Members of the presynaptic neurexin (NRX) and postsynaptic neuroligin (NL) transmembrane protein families form the axis of a signaling pathway that is crucial for the formation and function of excitatory and inhibitory synapses throughout the brain. MDGA proteins bind NLs and control their function and interaction with NRXs via unknown mechanisms. MDGA proteins are attached to the postsynaptic membrane via a C-terminal GPI anchor, and their large (∼900 amino acids) extracellular domain consists of six immunoglobulin-like domains (Ig1-6), a fibronectin type III-like (FnIII7) domain, and a memprin, A5, mu (MAM8) domain. The extracellular region of the NLs contains a cholinesterase-like domain that forms a stable interaction with the α/β-NRX1-3 LNS6 (laminin, NRX, sex-hormone-binding globulin) domain (Araç et al., 2007, Chen et al., 2008, Fabrichny et al., 2007).

We performed an extensive crystallization screening of the NL-MDGA complexes formed between MDGA1-2ECTO and NL1-2ECTO constructs from various species, and succeeded in generating diffraction-quality crystals and determining the structure of the Endo F1-treated complex formed between cMDGA1ECTO and the human NL1 cholinesterase domain lacking splice inserts (hNL1ECTO; Gln46-Asp635) at 3.30 Å. The hNL1ECTO-cMDGA1ECTO complex has a 2:2 stoichiometry and overall dimensions of ∼180 Å wide, ∼110 Å high, and ∼120 Å deep. Two MDGA1 monomers flank the NL1 dimer to form a 2-fold symmetric complex. The NL1 and MDGA1 C termini point in the same direction and thus confirm an interaction in cis, situated on the postsynaptic membrane. Each MDGA1 molecule spans the NL1 dimer using two large, separate interaction sites located on both NL1 monomers (Sites I and II). The Ig1-3 domains mediate all MDGA1 contacts, consistent with previous domain-deletion experiments (Pettem et al., 2013). The smaller Site I (859 Å2 BSA) is formed between residues from (1) MDGA1Ig1 β strands C, F, and G and loop CE and (2) NL1 loops Leu289-Gln307, Ile377-Asp385 (part of “loop L1”), Gln392-Tyr398, and Phe496-Pro499 and helices α2(4,5) and α4(6,7). The larger Site II (1,000 Å2 BSA) is formed between residues from MDGA1Ig2 β strands A, B, D, and E and NL1 α helices α2(7,8) and α3(7,8); (2) MDGA1Ig2 loop ABIg2 and NL1 loops Ala110-Pro132 (“Cys loop”) and Asp361-Asp385 (“loop L1”); and peripheral interactions contributed by MDGA1Ig3 to NL1 α helix α2(7,8) and loop Val417-Ser424. The PheNL1430-PheMDGA1154 π-π sandwich stacking interaction is central to this interface and is lined by multiple hydrogen-bonding and charged interactions. Furthermore, the LRE motif is present in the majority of mammalian AChEs, and besides in NL, it is also observed in the cholinesterase-like adhesion molecules neurotactin and glutactin. Both Arg450 and Glu451 form an integral part of the NL-MDGA interface and interact with Tyr187 and Leu190, respectively, on MDGA1 loop DEIg2, offering a first functional role for this LRE-tripeptide in NLs.

> TGQKLDDVDPLVATNFGKIRGIKKELNNEILGPVIQFLGVPYAAPPTGERRFQPPEPPSPWSDIRNATQFAPVCPQNIIDGRLPEVMLPVWFTNNLDVVSSYVQDQSEDCLYLNIYVPTEDDIRDSGGPKPVMVYIHGGSYMEGTGNLYDGSVLASYGNVIVITVNYRLGVLGFLSTGDQAAKGNYGLLDLIQALRWTSENIGFFGGDPLRITVFGSGAGGSCVNLLTLSHYSEGLFQRAIAQSGTALSSWAVSFQPAKYARMLATKVGCNVSDTVELVECLQKKPYKELVDQDIQPARYHIAFGPVIDGDVIPDDPQILMEQGEFLNYDIMLGVNQGEGLKFVENIVDSDDGISASDFDFAVSNFVDNLYGYPEGKDVLRETIKFMYTDWADRHNPETRRKTLLALFTDHQWVAPAVATADLHSNFGSPTYFYAFYHHCQTDQVPAWADAAHGDEVPYVLGIPMIGPTELFPCNFSKNDVMLSAVVMTYWTNFAKTGDPNQPVPQDTKFIHTKPNRFEEVAWTRYSQKDQLYLHIGLKPRVKEHYRANKVNLWLELVPHLHNLNDRTKHHHHHH;> QGVYAPAQAQIIHAGQACVVKEDNISERVYTIREGDTLVLQCLVTGHPRPQVRWTKTAGSASDKFQETSVLNETLRIEKIQRLQGGRYYCKAENGVGVPAIKSIRVDVQYLDEPVLTVHQTISDVRGSFYQEKTVFLRCTVNSNPPARFIWKRGAETLSHSQDNGVDIYEPLYTQGETKVLKLKNLRPQDYASYTCQVSVRNVCSIPDKSITFQLTNTTAPPALKLSVNETLVVNPGDNVTMQCSLTGGDPQPEVLWSHSPGPLPPNSLVQGGNLTIWRIRVEDSGYYNCTAINNVGNPAKKTVNLLVRSMKNATFQITPDVIKESETIQLGQDLKLSCHVDAVPQEKVVYSWYKNGKPARFSDRLLITRNDPELPPVTCSLEIIDLRFSDYGTYLCVATFQGAPIPDLSVEVNISSETVPPTISVPKGQSTITVREGSRAELQCEVRGKPKPPIIWSRVDKETPMPSGTMTVETYDGKLRLESVSRDMSGTYKCQTARYNGFNIRPREALVQLNVQFPPVVEPAFQDVRQGMGRSVTLRCTMLKGSPMKVATSVWRFNGTLLAQPPAEQQDYSELKVDSVSRETSGSYECSISNDVGVSACLFQVSAKAYSPEFYYDTPNPTLSQKQSKNYSYILQWTQKEPDAVDPILKYRLEVRQLAQRNTIQTFIPVQKMEKGLLLEHILPNLKVPQSYEVRLTPITSFGAGDMAARIIRYMEPINYPSPTDNTCRFEDEKICGFVQDKMDNFDWTRQNALTQNPKRTVNTGPPTDISGTPEGYYMFIEASRPRVTGDKARLISPLYNITAKYYCVSFYYHMYGKHIGSLNLLVRVRNKRAIDTQVWSLSGNRGNMWQQAHVPINPPGPFQIIFEGVRGTSYEGDIAIDDVTLKKGDCPRKPIGPNKGTKHHHHHH> MIAEFIDGLQKFHFLQNALITAIVVGIVAGAVGCFIILRGMSLMGDAISHAVLPGVALSFILGLDFFIGAIVFGLLAAIIITY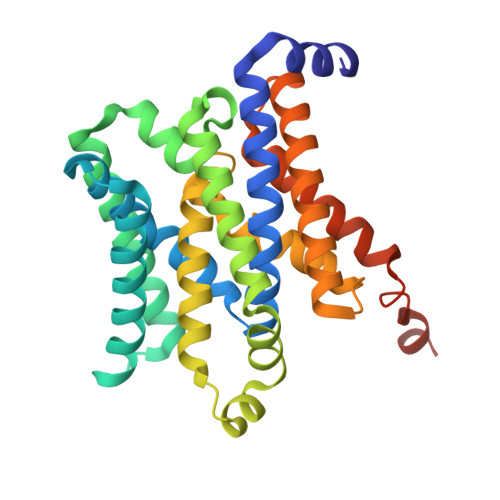IKGNSIIKSDTAIGITSSSFLALGIILIGVAKSSTDLFHILFGNILAVQDTDMFITMGVGAAILLLIWIFFKQLLITSFDELLAKAMGMPVNFYHYLLMVLLTLVSVTAMQSVGTILIVAMLITPAATAYLYANSLKSMIFLSSTFGATASVLGLFIGYSFNVAAGSSIVLTAASFFLISFFIAPKQRYLKLKNKHLLKGSENLYFQ> TKLHNTIFSETRKFTRESFKEIEHLTARLANDRVARHDFLFNTSIVLISDYSGEDSNGNQLQATITIPNEIINPKEYDPSDYPLAEDESFFKQGHKYDYLVTFRAGSLTNTYEPKTKMYKLHAALDKLMHVKQRKSRFADLWRELCAVIASLDVWYQTTNYPLRTYVKLLFHKGDEFPFYESPSQDRIIFNDKSVASILPTFVYTCCQVGTAIMSGILTHVESIVAMNHFLHCAKDSYIDEKLKIKGIGRSWYQEALHNVCQATVPV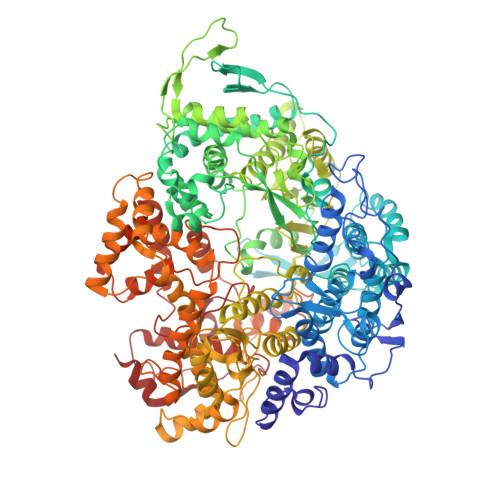WSQFNEVIGHRTKSTSEPHFVSSTFISLRAKRAELLYPEFNAYINRAIQLSKTQNDVANYYAACRAMTNDGTFLATLTELSLDAAVFPRIEQHLVTRPAVLMSNTRHESLKQKYTNGVGSIAQSYLSSFTDEIAKRVNGRHHDEAWLNFLTTSSPGRKLTEIEKLEVGGDVAAWSNSRIVMQAVFAREYRTPERIFKSLKAPIKLVERQQSDRRQRAISGLDNDRLFLSFMPYTIGKQIYELNDNAAQGKQAGNAFDIGEMLYWTSQRNVLLSSIDVAGMDASVTTNTKDIYNTFVLDVASKCTVPRFGPYYAKNMEVFEAGNRQSQVRYVNAAWQACALEAANSQTSTSYESEIFGQVKNAEGTYPSGRADTSTHHTVLLQGLVRGNELKRASDGKNSCLATIKILGDDIMEIFQGSESDTYDHAVSNASILNESGFATTAELSQNSIVLLQQLVVNGTFWGFADRISLWTREDTKDIGRLNLAMMELNALIDDLVFRVRRPEGLKMLGFFCGAICLRRFTLSVDNKLYDSTYNNLSKYMTLTKYDKNPDSDSTLMSLILPLAWLFMPRGGEYPAYPFERRDGTFTEDESMFTARGAYKRRLLYDVSNIGEMIQQNSMALDDDLLHEYGFTGALLLIDLNILDLIDEVKKEDISPVKVSELATSLEQLGKLGEREKSRRAASDLKIRGHALSNDIVYGYGLQEKIQKSAMATKETTVQSKRVSSRLHDVIVAKTRDYKISTIPADALHLHEFEVEDVTVDLLPHAKHTSYSSLAYNMSFGSDGWFAFALLGGLDRSANLLRLDVASIRGNYHKFSYDDPVFKQGYKIYKSDATLLNDFFTAISAGPKEQGILLRAFAYYSLYGNVEYHYVLSPRQLFFLSDNPVSAERLVRIPPKYYVSTQCRALYNIFSYLHILRSIANNRGKRLKMVLHPGLIAYVRG>[2x]VTERPRDCRPVVRRA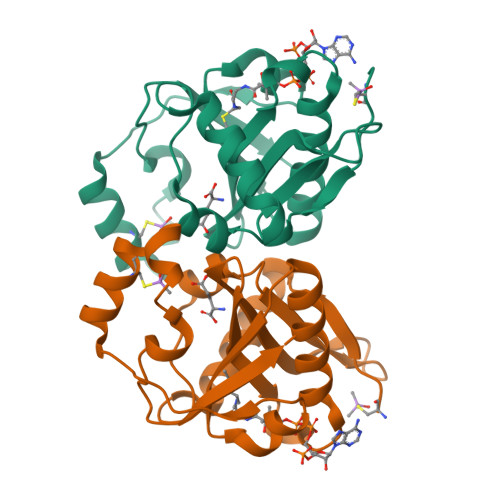RTSDVPAIKQLVDTYAGKILLEKNLVTLYEAVQEFWVAEHPDLYGKVVGCGALHVLWSDLGEIRTVAVDPAMTGHGIGHAIVDRLLQVARDLQLQRVFVLTFETEFFARHGFTEIEGTPVTAEVFDEMCRSYDIGVAEFLDLSYVKPNILGNSRMLLVL>[8x]SNATLRIAAMPALANGLLPRFLAQFIRDRPNLQVSLMGLPSSMVMEAVASGRADIGYADGPQERQGFLIETRSLPAVVAVPMGHRLAGLDRVTPQDLAGERIIKQETGTL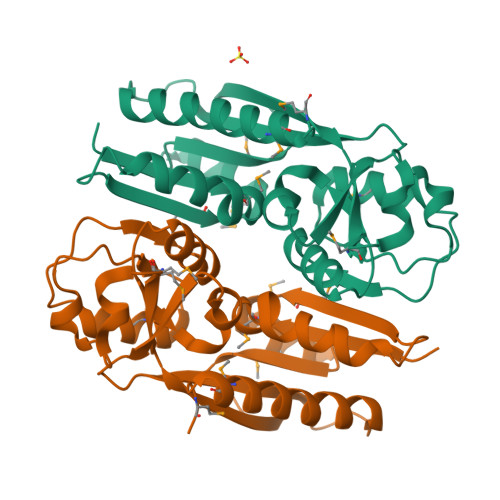FAMRVEVAIGGIQRRPSIEVSLSHTALSLVREGAGIAIIDPAAAIEFTDRIVLRPFSIFIDAEFLEVRSAIGAPSTIVDRFTTEFWRFHDDLMKQNGLME>MPQDPSTRSSPARLLI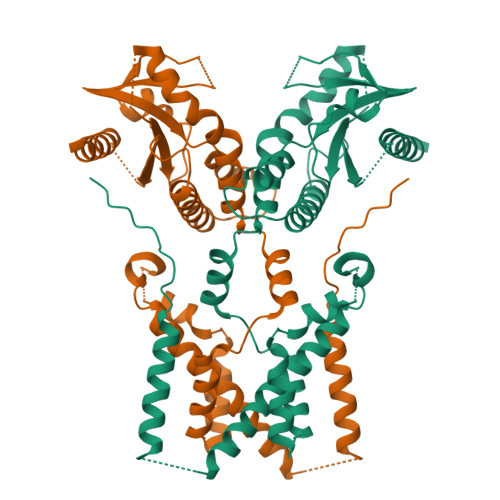PEPRAGRARHAACVLLAVCFVVLFLSGEPLAPIIRSVCTQLAALQLGVLLKGCCCLAEEIFHLHSRHHGSLWQVLCSCFPPRWYLALLLVGGSAYLDPPEDNGHSPRLALTLSCLCQLLVLALGLQKLSAVEVSELTESSKKNVAHGLAWSYYIGYLKVVLPRLKECMEELSRTNPMLRAHRDTWKLHILVPLGCDIWDDLEKADSNIQYLADLPETILTRAGIKRRVYKHSLYVIRDKDNKLRPCVLEFASPLQTLCAMSQDDCAAFSREQRLEQARLFYRSLRDILGSSKECAGLYRLIAYEEPAEPESHFLSGLILWHLQQQQREEYMVQEELPLGTSSVELSLQVSSSDLPQPLRSDCPGIHRPDYKDDDDK[2x]>GPGSMQPSPDSPAPLNVTVPFDSELGLQFTELGPDGARAQLDVRPKLLQLTGVVHGGVYCAMIESIASMAAFAWLNSHGEGGSVVGVNNNTDFVRSISSGMVYGTAEPLHRGRRQQLWLVTITDDTDRVVARGQV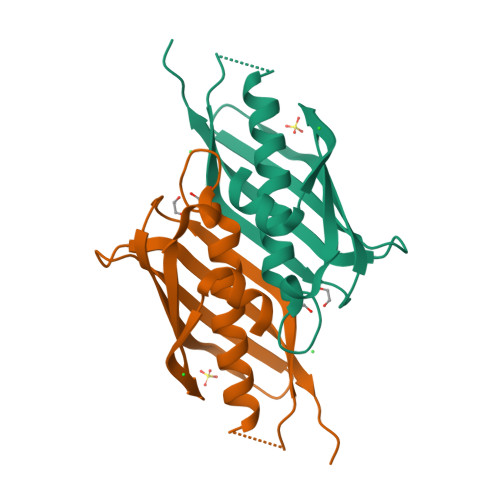RLQNLEARP[2x]> QGMNTIESITADLHGLGVRPGDLIMVHASLKAVGPVEGGAASVVSALRAAVGSAGTLMGYASWDRSPYEETLNGARMDEELRRRWPPFDLATSGTYPGFGLLNRFLLEAPDARRSAHPDASMVAVGPLAATLTEPHRLGQALGEGSPLERFVGHGGKVLLLGAPLDSVTVLHYAEAIAPIPNKRRVTY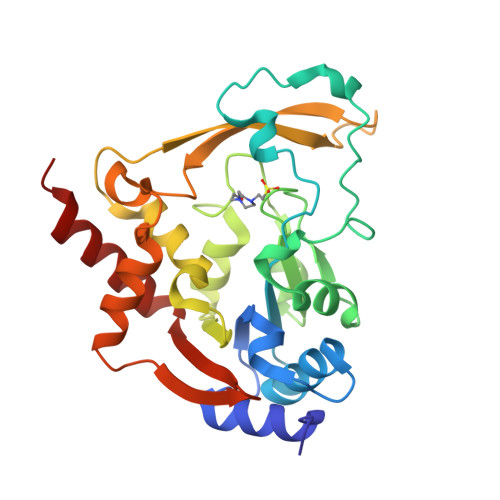EMPMLGPDGRVRWELAEDFDSNGILDCFAVDGKPDAVETIAKAYVELGRHREGIVGRAPSYLFEAQDIVSFGVTYLEQHFGAP> MKMDKKTIVWFRRDLRIEDNPALAAAAHEGSVFPVFIWCPEEEGQFYPGRASRWWMKQSLAHLSQSLKALGSDLTL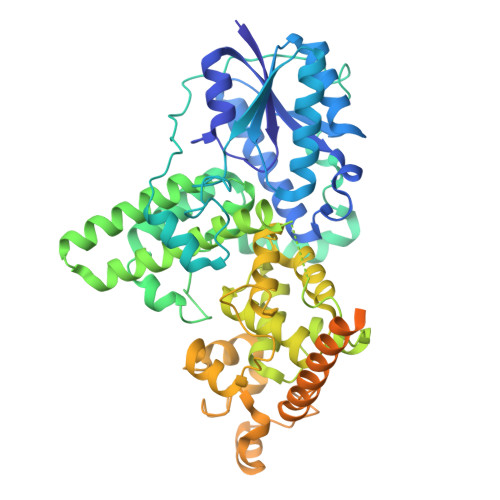IQTHNTISAILDCIRVTGPTKVVFNHLYDPVSLVRDHTVKEKLVERGISVQSYNGDLLYEPWEIYCEKGKPFTSFNSYWKKCLDMSIESVMLPPPWRLMPITAAAEAIWACSIEELGLENEAEKPSNALLTRAWSPGWSNADKLLNEFIEKQLIDYAKNSKKVVGNSTSLLSPYLHFGEISVRHVFQCARMKQIIWARDKNSEGEESADLFLRGIGLREYSRYICFNFPFTHEQSLLSHLRFFPWDADVDKFKAWRQGRTGYPLVDAGMRELWATGWMHNRIRVIVSSFGVKFLLLPWKWGMKYFWDTLLDADLECDILGWQYISGSIPDGHELDRLDNPALQGAKYDPEGEYIRQWLPELARLPTEWIHHPWDAPLTVLKASGVELGTNYAKPIVDIDTARELLAKAISRTREAQIMIGAAPDEIVADSFEALGANTIKEPGLCPSVSSNDQQVPSVVRYNGSKRVKPEEEEERDMKKSRGFDERELFSTAESSSSSSVFFVSQSCSLASEGKNLEGIQDSSDQITTSLGKNGCK Eukaryotic translation initiation factor 2B (eIF2B) is the decameric guanine nucleotide exchange factor (GEF) for the GTPase eukaryotic translation initiation factor 2 (eIF2). Upon delivery of the initiator Met-tRNAi to the site of translation initiation, bound GTP is hydrolyzed and eIF2 is released from the scanning ribosome. eIF2B catalyzes GDP-GTP exchange on eIF2, enabling rebinding of Met-tRNAi to allow for a new cycle of mRNA translation initiation. Two catalytic subcomplexes, each comprised of a γ and ε subunit, decorate the central regulatory core, which is a heterohexamer composed of two α, β and δ subunits. Curiously, the eIF2B regulatory core is related to an ancient family of homo-hexameric sugar phosphate-metabolizing enzymes, with conservation observed between eIF2Bα/β/δ and the archaeal ribose-1,5-bisphosphate isomerase (RBPI).

Motivated by our biochemical evidence that sugar phosphates are activators of eIF2B, we determined a 2.9 Å cryo-EM structure of eIF2B bound to F6P, the highest affinity identified ligand. The eIF2B-F6P complex shares the same overall architecture as previously reported eIF2B structures. F6P occupies an inter-domain cavity within each eIF2Bα monomer (chains G and H), which is the conserved metabolite binding pocket in the ancestral eIF2Bα/β/δ homologs. This pocket is on the opposite face of the eIF2B holoenzyme from the previously described ISRIB binding pocket that sits at the symmetric eIF2Bβ/δ interface. Protein-ligand interactions in the F6P pocket are mediated by both the sugar and phosphate moieties. G196, A129, Y130, E198, and N208 form H-bonds with the F6P pyranose ring, while the positively charged residues R132 and K234 coordinate the phosphate group. The 1′ position of F6P is exposed to solvent, suggesting a way by which bulkier ribonucleotides (e.g. UMP and AMP) could be accommodated in this site. Notably, we did not observe electron density for any ligands within the eIF2Bβ or eIF2Bδ metabolite pockets, despite their homology to eIF2Bα. The holoenzyme structures in the absence and presence of F6P are also strikingly similar, with global r.m.s.d. = 1.6 Å. The most prominent difference is a uniform shift in the position of both eIF2Bε subunits, wherein the β-sheet rich domain moves inwards towards the cognate eIF2Bα subunit by ~1.5–2 Å.

>MAAPVVAPPGVVVSRANKRSGAGPGGSGGGGARGAEEEPPPPLQAVLVADSFDRRFFPISKDQPRVLLPLANVALIDYTLEFLTATGVQETFVFCCWKAAQIKEHLLKSKWCRPTSLNVVRIITSELYRSLGDVLRDVDAKALVRSDFLLVYGDVISNINITRALEEHRLRRKLEKNVSVMTMIFKESSPSHPTRCHEDNVVVAVDSTTNRVLHFQKTQGLRRFAFPLSLFQGSSDGVEVRYDLLDCHISICSPQVAQLFTDNFDYQTRDDFVRGLLVNEEILGNQIHMHVTAKEYGARVSNLHMYSAVCADVIRRWVYPLTPEANFTDSTTQSCTHSRHNIYRGPEVSLGHGSILEENVLLGSGTVIGSNCFITNSVIGPGCHIGDNVVLDQTYLWQGVRVAAGAQIHQSLLCDNAEVKERVTLKPRSVLTSQVVVGPNITLPEGSVISLHPPDAEEDEDDGEFSDDSGADQEKDKVKMKGYNPAEVGAAGKGYLWKAAGMNMEEEEELQQNLWGLKINMEEESESESEQSMDSEEPDSRGGSPQMDDIKVFQNEVLGTLQRGKEENISCDNLVLEINSLKYAYNISLKEVMQVLSHVVLEFPLQQMDSPLDSSRYCALLLPLLKAWSPVFRNYIKRAADHLEALAAIEDFFLEHEALGISMAKVLMAFYQLEILAEETILSWFSQRDTTDKGQQLRKNQQLQRFIQWLKEAEEESSEDD[2x];>[2x]MDYKDDDDKENLYFQSMPGSAAKGSELSERIESFVETLKRGGGPRSSEEMARETLGLLRQIITDHRWSNAGELMELIRREGRRMTAAQPSETTVGNMVRRVLKIIREEYGRLHGRSDESDQQESLHKLLTSGGLNEDFSFHYAQLQSNIIEAINELLVELEGTMENIAAQALEHIHSNEVIMTIGFSRTVEAFLKEAARKRKFHVIVAECAPFCQGHEMAVNLSKAGIETTVMTDAAIFAVMSRVNKVIIGTKTILANGALRAVTGTHTLALAAKHHSTPLIVCAPMFKLSPQFPNEEDSFHKFVAPEEVLPFTEGDILEKVSVHCPVFDYVPPELITLFISNIGGNAPSYIYRLMSELYHPDDHVL;>MAAVAVAVREDSGSGMKAELPPGPGAVGREMTKEEKLQLRKEKKQQKKKRKEEKGAEPETGSAVSAAQCQVGPTRELPESGIQLGTPREKVPAGRSKAELRAERRAKQEAERALKQARKGEQGGPPPKASPSTAGETPSGVKRLPEYPQVDDLLLRRLVKKPERQQVPTRKDYGSKVSLFSHLPQYSRQNSLTQFMSIPSSVIHPAMVRLGLQYSQGLVSGSNARCIALLRALQQVIQDYTTPPNEELSRDLVNKLKPYMSFLTQCRPLSASMHNAIKFLNKEITSVGSSKREEEAKSELRAAIDRYVQEKIVLAAQAISRFAYQKISNGDVILVYGCSSLVSRILQEAWTEGRRFRVVVVDSRPWLEGRHTLRSLVHAGVPASYLLIPAASYVLPEVSKVLLGAHALLANGSVMSRVGTAQLALVARAHNVPVLVCCETYKFCERVQTDAFVSNELDDPDDLQCKRGEHVALANWQNHASLRLLNLVYDVTPPELVDLVITELGMIPCSSVPVVLRVKSSDQ[2x];>[2x]MDDKELIEYFKSQMKEDPDMASAVAAIRTLLEFLKRDKGETIQGLRANLTSAIETLCGVDSSVAVSSGGELFLRFISLASLEYSDYSKCKKIMIERGELFLRRISLSRNKIADLCHTFIKDGATILTHAYSRVVLRVLEAAVAAKKRFSVYVTESQPDLSGKKMAKALCHLNVPVTVVLDAAVGYIMEKADLVIVGAEGVVENGGIINKIGTNQMAVCAKAQNKPFYVVAESFKFVRLFPLNQQDVPDKFKYKADTLKVAQTGQDLKEEHPWVDYTAPSLITLLFTDLGVLTPSAVSDELIKLYLGGENLYFQAEDKGGGSGGGGSGGGGSASQGGLNDIFEAQKIEWHEGGGGSGGGGSGGGGSGRDQDYKDDDDK;>[2x]MEFQAVVMAVGGGSRMTDLTSSIPKPLLPVGNKPLIWYPLNLLERVGFEEVIVVTTRDVQKALCAEFKMKMKPDIVCIPDDADMGTADSLRYIYPKLKTDVLVLSCDLITDVALHEVVDLFRAYDASLAMLMRKGQDSIEPVPGQKGKKKAVEQRDFIGVDSTGKRLLFMANEADLDEELVIKGSILQKHPRIRFHTGLVDAHLYCLKKYIVDFLMENGSITSIRSELIPYLVRKQFSSASSQQGQEEKEEDLKKKELKSLDIYSFIKEANTLNLAPYDACWNACRGDRWEDLSRSQVRCYVHIMKEGLCSRVSTLGLYMEANRQVPKLLSALCPEEPPVHSSAQIVSKHLVGVDSLIGPETQIGEKSSIKRSVIGSSCLIKDRVTITNCLLMNSVTVEEGSNIQGSVICNNAVIEKGADIKDCLIGSGQRIEAKAKRVNEVIVGNDQLMEI(2R)-N-{(2S,3R)-4-{[(4'S)-6'-(2,2-dimethylpropyl)-3',4'-dihydrospiro[cyclobutane-1,2'-pyrano[2,3-b]pyridin]-4'-yl]amino}-3-hydroxy-1-[3-(1,3-thiazol-2-yl)phenyl]butan-2-yl}-2-methoxypropanamide | C33 H44 N4 O4 S | 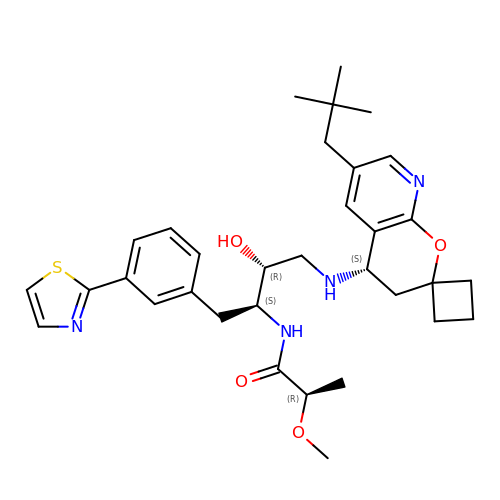IUSARDYWEPUTPN-OZBXUNDUSA-N> ATGYDAVDDLLHYHERGNGIQINGKDSFSNEQAGLFITRENQTWNGYKVFGQPVKLTFSFPDYKFSSTNVAGDTGLSKFSAEQQQQAKLSLQSWADVANITFTEVAAGQKANITFGNYSQDRPGHYDYGTQAYAFLPNTIWQGQDLGGQTWYNVNQSNVKHPATEDYGRQTFTHEIGHALGLSHPGDYNAGEGNPTYNDVTYAEDTRQFSLMSYWSETNTGGDNGGHYAAAPLLDDIAAIQ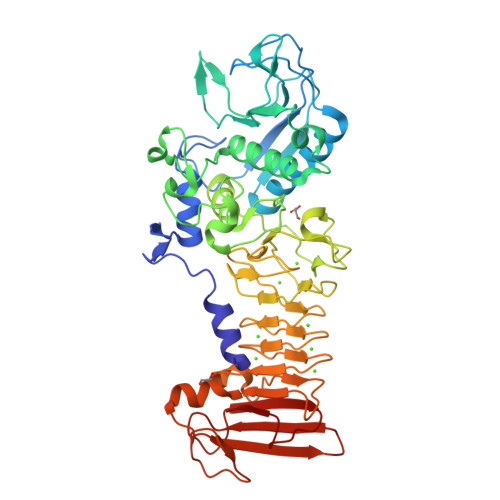HLYGANLSTRTGDTVYGFNSNTGRDFLSTTSNSQKVIFAAWDAGGNDTFDFSGYTANQRINLNEKSFSDVGGLKGNVSIAAGVTIENAIGGSGNDVIVGNAANNVLKGGAGNDVLFGGGGADELWGGAGKDIFVFSAASDSAPGASDWIRDFQKGIDKIDLSFFNKEANSSDFIHFVDHFSGTAGEALLSYNASSNVTDLSVNIGGHQAPDFLVKIVGQVDVATDFIV> PLVWTQLKQTGTTQPTARSGHTIITVGKTHIMFGGLDNDKNNYKDGKIAPNNQVFTLKLTQNNCEWRQIACQGDVPLPRCYHASCAISADKMLVFGGSYTSNLRFNDTYILKTTSYQWSKPANQISGGEPKNAESKIGAPQPRYGHSATFFEGKVYIFGGHGGINYQRLAFNDLYVLETENFEWTRLEPKGNPPDPRGGHSAAMMANKPQLMIFGGWSFTSQYSNIMIYDIEKDEWVDPEIAHEIPKWNLSGIMAPSIPSWKYFIFGGSVGSFEEGGNRTNSRFVDDSFVLDIDTLSWSSINLEADETSKAVCKPRPRESASIFYDSGESRAIVFGGWANNWLNDLWALNVSTITGPPIFSIKPALGPLTGKTKVLIEGDGFKDTQNISVKFSGGKLEKEVNGTFVNEKEISCETPTFDYPRSVEVTVCMNKGDYTITKSAFTYNTKADKTIAYGPGLLTENLIGVQTTIVIQARNGSDEFVVTIRNPAKIKKEEEVKEGDKANTKNTIKEDEEEEGEDEEENKKKKEAEKNDLTGSAVMNYISKQLKDIQEFIENTKENIEIRNKNISELINVMINLEKVRVKNDDDVLTLDTVEEMLNFLKKKKDSDIKKCKKLQEEWKNLAKMAQAVKKDIQNPVKTESDKTKENIKKFEEITLKEYANSLKKESFFIYKTGVSESFKRIGEVKQKVDEFEVQLNQYEDFARIGSKKLMEQIRTDVSSVEKLWVRIEISEKTMDEYKKMKWGSINSMDMEDEIKKLRKALTDLRGIDKRSNAFIGITEELKKWATFLPLLGELKDPSMNSEDGRHWKKLKDLVKKEFDVSQELMLEIIWDLKLFDYKDGIEEITDQAKQELKMEKALKKIIDFWRDIEFELVQHKNTDIHTLKMSEENFETLEDHQLQINNMLLSKYVAYFEKEVEKWKYDLGSVYDVVQLLLEVQKTWSFLENLFEVKRELPNESAQFVGIDKDMKEIMQKGCDIKNCLKFCTIEGMLKRLENIQAQLKVCEKALNEFLDSKRRAFPRFYFVSVNDLLDILSNGNSPAKINRHMSKIFQAIDNLQLKEDSSGGRPTLKMISCVGTEEVDFSSPRLLQGKVESYLKDVIDTMIGTLKSVANSSFKNFQSMTRKEWLKSDPSQITLLVNNIIWSKAVEDCFLKLQSGDINAMKLFLDESIKQLTELIGMVQGDLSKPLRQKIMCLITIDTHSRDVVHRLINEHVRKAEEFQWQSQLKFYWVDNDAKIKIADARFVYNYEYLGNGPRLVITPLTDRIYVTATQALHLKMGCAPAGPAGTGKTETTKDLANALAKACYVFNCSSEMNYESMGNIYKGLASSGCWGCFDEFNRLLPEVLSVCSVQFKAVTDAIKQNVERFIIEGDEISLDPTCGVFITMNPGYLGRAELPEGLKALFRPITVVVPDLELICENMLMAEGFIEAKILAKKFVTLYMLCRDLLSKQLHYDWGLRAIKSVLVVAGGFKRSEPEIAEQALLMRALRDFNIPKIAFQDLYVFHGLLGDLFPGINIKPKKDLDFEKIITDVCIENKLDPDPEFVLKVVQLSELLAIRHCVFVMGPPGAGKSTTWKILAKAQDKTNKKTTLIDIDPKVVSTKDFYGYNLPSKEWKDGLFSKMLRSLAEQPDTNPKWICLDGDLDANWIESMNSVMDDNKILTLANNERIPLKPHMRALFEIRDLRFATPATVSRAGILYISDEVGYQWRSYVKSWIKQEFSQDQEMSKNLDTLFGKYVPDTLDHIKKHCRFLVPVSPISQVISICKSLQTLLKGDVKNLEYLFVYALIWAIGGALAEKDSIDYRKDFSTWWKGAWKTAVKFPSKGTIFDYYVDQSGDSSKFVEWSKRLENKEFDPQVETMGNITVNTIETLATTEFIKSYLMVKHPSLLIGNSGCGKTQLAKGILKEIVQAKPENYAYQLINFNYYTDSTYLQGQIEQTLEKKAGRQYGPPGKVQLIYFIDDLNMPQLDAYDTQTAIALLRQLADYGHFYDVSKLALKDIINTQVLAAMNPSAGSFFVNPRYQRHFWTISIPFPDNESLSLIYITFLNGHLKRFKSTIQEYSNIIVRASLMLHQAVTQNFRKTAINFHYEFNLRHMSNVFQGLLLSDPNKFTE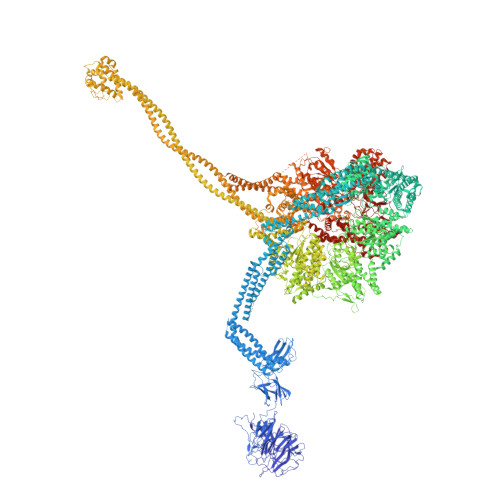PDKLIKLWIHECERTYGDRLVSTDNLKTYKENIFDIVKKSFSKFNFSRYFGNNPENLIYCNFIAGINSDRFYDQMPNNEMEKHISEALKEYNDNNAFMGLVLFEDAMKHVCRICRIVLPSSGHALLVGVGGSGKQSLSKLASFIMGYTTFSITISATYSMVDLRNDLQQLYFKCGPKEEGILFLFTEGQITNERFLVYINDLLSSGEIAELYTLDEKEAMINQVRAKVKGEGKPDTRENCWNWFIDQVKKNLHMAICFSPVGDMRRRARQFPALVNCTVIDWFQPWPYEALFNVAKSFLEPVDLGDDKVREAVVKFMPFSFTLVNDLGLKLLEQERRYAYTTPKSFLELISLFTNMLAQKRESLERNKERYETGLVKLKETAEQVAIIEVEVKEKQVEAEAKKKEADAFAEVVGREKDKVEKENSKATIEADKCGLIKQNVEAQKSSTQQDLDAAQPLVEQAKSALNSISKKDFQQAKSFASPPAGVPEVFAATIYLLAGYFNEAIEIDKNKKPKDVSWKSSLKLMKSPEEFMEKLLNFKDVVDANQVANVNIVKNQYLNMPSFTPEQMASKSAAAKGICSWVVNIVKYYDVIQDVEPKRKALKEATEQLEEATVKLNEVEEVVRKLNEELNKLKAENDKAIAERNAAISEAERCARRLNLAQRLVTALSSENERWGKSIIQLEDQLKLMVGDVLVASSFVSYSGPFNKKFRNIMINQNFMKFMKEHTIPMSPDPNPIKILTDESTIALWNKQKLPSDSVSIENGTILTNSARYPLMIDPQLQGITWIREKEKANNLKILRLGSKNINRDLELSIENGYSAIIENMNERIDAILMPIIARSFIKRGKNKIIKFAGKDLILHPNFKLFLHTKLSNPHYPPEIQAEAALINFTVTEAGLGDQLLSLVVARERPDLAKMKIELITQQNDFKIKLKDLEDELLYKLANAKGDILDDIELIENLEYSKKLSVEIAEKVAAAKITEAKINETSENYRPAASRGALFYFLLSDLSKVHSFYKYSLESFIVVINRAIDAISENKIYGKTTMMSPRSLKKRVDELIESLTYTAYQTTRRGLFESHKLIVAAMLCLRVLLRSEELNSDEVDHLIIGKVDVNPTPMPDALKSFLNDNIWAACKALETIHQFQGFCQSLETDVLQWKKWYSEEKAETADLPKAFKELSKFHRLLLLRALRPDRLPSALSQFVHDKMGERYIEQPPFNIFETFQETSKTVPIFFVLFPGVDPTPDVERVAATFDVSANNGRFINISMGQGQEDRAKKALFDCAQKGHWIMLQNVHLMQSWLYGLNGLEGFLESVFASPKTHPNFRVFISSEPPNVLLPLMQIIPESILQGSLKIANEAPQYLKANLRRAYNKFDQEFLDKCDKKPTEFKSCLFALCFFHSLMLGRKKFGTQGWSRVYNFNDGDLTICADVLYNYLSKYDQVPWDDLRYIFGEIMYGGHITDDWDRRTNRTYLKVLIRSELLQQNFNLAPQFKSPDPSKFDYEAYRKYIEEKLPIESPQMFGMHPNAEIGYLTQTCDQVFNTILEVQGGSSGGGASKKDDGVMVTLTDFKTRCPHDFNMLLIEEKVKEKTPYIVVCLQECERMNGLLKEIKTSLEDLRLGLTGALNMTDAMESLQQSLSFNKVPDTWEKKAYFSKKPLSSWFADLIERNIQLQEWCKELVTPTSLCISYLFNPMSYLTAIMQFTARAQGLPLDGITIQTNVTAMKGPEDVVNPAENGAYIHGLFLEGAAWEIGGQGQDGYLIEQKPKELHPKMPVINAVAVPLDKKKKNGQYDCPTYVTSARGQTFVFTANLNMESDDSDPNKWILSGTCMLMSDD>MSLHYQPKQDLLNDRIILVTGASDGIGREAAMTYARYGATVILLGRNEEKLRQVASHINEETGRQPQWFILDLLTCTSEDCQQLAQRIAVNYPRLDGVLHNAGLLGDVCPMSEQDPQVWQDVMQVNVNATFMLTQALLPLLLKSDAGSLVFTSSSVGRQGRANWGAYAASKFATEGMMQVLADEYQQRLRVNCINPGGTRTAMRASAFPTEDPQKLKTPADIMPLYLWLMGDDSRRKTGMTFDAQPGRKPGISQEGHHHHH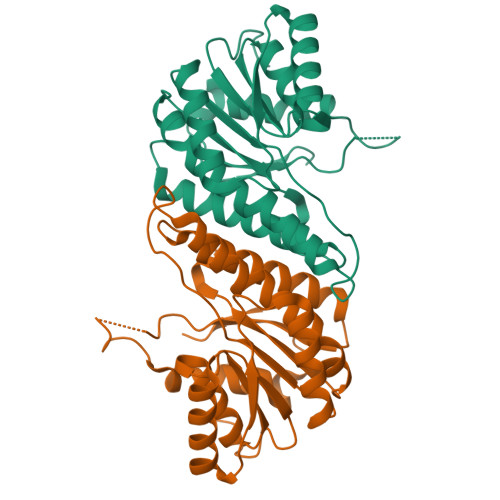H[2x]>MDPFLVLLHSVSSSLSSSELTELKFLCLGRVGKRKLERVQSGLDLFSMLLEQNDLEPGHTELLRELLASLRRHDLLRRVDDFEAGAAAGAAPGEEDLCAAFNVICDNVGKDWRRLARQLKVSDTKIDSIEDRYPRNLTERVRESLRIWKNTEKENATVAHLVGAL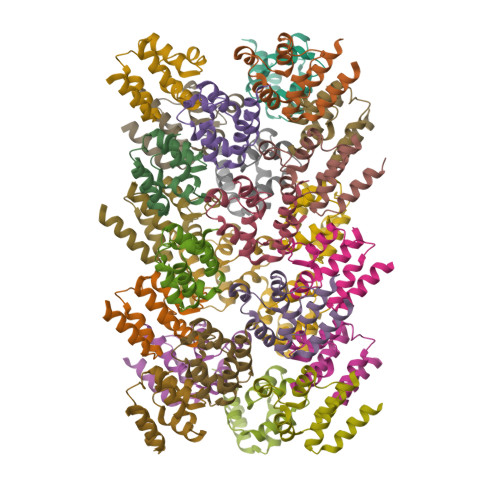RSCQMNLVADLVQEVQQARDLQNRSGAMSPMSWNSDASTSEAS[24x]> GSPPGPPGGVVVRDIGDTTVQLSWSRGFDNHSPIAKYTLQARTPPSGKWKQVRTNPVNIEGNAETAQVLGLMPWMDYEFRVSASNILGTGEPSGPSSRIRTKEAVPSVAPSGLSGGGGAPGELTINWTPMSREYQNGDGFGYLLSFRRQGSS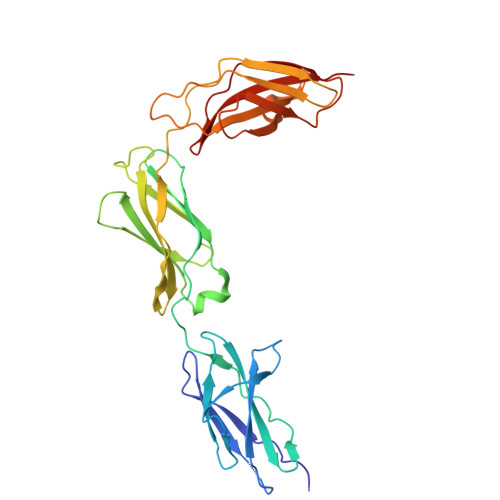SWQTARVPGADTQYFVYSNDSIHPYTPFEVKIRSYNRRGDGPESLTAIVYSAEEEPKVAPAKVWAKGSSSSEMNVSWEPVLQDMNGILLGYEIRYWKAGDKEAAADRVRTAGLDSSARVTGLYPNTKYHVTVRAYNRAGTGPASPSADAMTMK4-(cyclohexylamino)pyrido[3,4-d]pyrimidin-8(7H)-one | C13 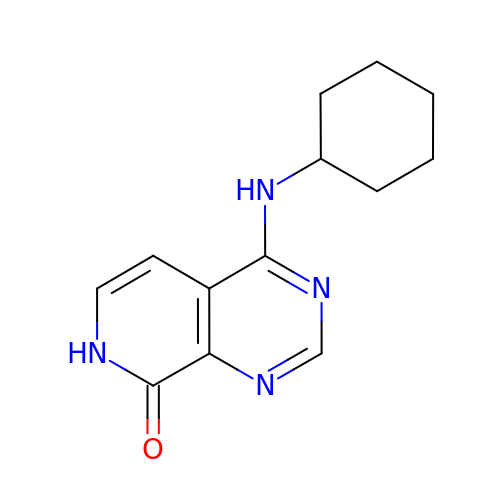H16 N4 O | FCTPOQHJQPWBOI-UHFFFAOYSA-N>PISPIETVPVKLKPGMDGPKVKQWPLTEEKIKALVEICTEMEKEGKISKIGPENPYNTPVFAIKKKDSTKWRKLVDFRELNKRTQDFWEVQLGIPHPAGLKKKKSVTVLDVGDAYFSVPLDEDFRKYTAFTIPSINNETPGIRYQYNVLPQGWKGSPAIFQSSMTKILEPFRKQNPDIVIYQYMDDLYVGSDLEIGQHRTKIEELRQHLLRWGLTTPDKKHQKEPPFLWMGYELHPDKWTVQPIVLPEKDSWTVNDIQKLVGKLNWASQIYPGIKVRQLCKLLRGTKALTEVIPLTEEAELELAENREILKEPVHGVYYDPSKDLIAEIQKQGQGQWTYQIYQEPFKNLKTGKYARMRGAHTNDVKQLTEAVQKITTESIVIWGKTPKFKLPIQKETWETWWTEYWQATWIPEWEFVNTPPLVKLWYQLEKEPIVGAETFYVDGAANRETKLGKAGYVTNRGRQKVVTLTDTTNQKTELQAIYLALQ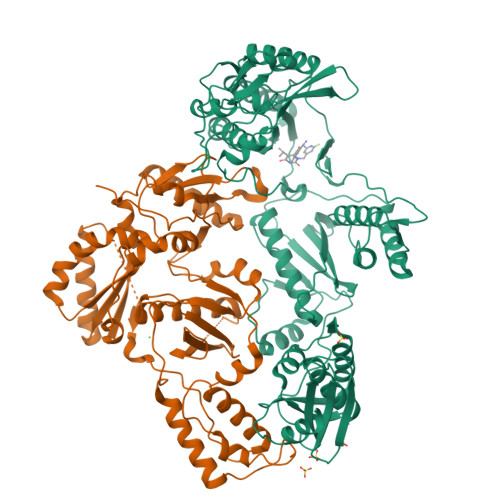DSGLEVNIVTDSQYALGIIQAQPDQSESELVNQIIEQLIKKEKVYLAWVPAHKGIGGNEQVDKLVSAGIRKVL[2x]>KRKIIYLASPYGFSQQQKTLLLPPIVRALEALGIEVWEPFARNNQIDFSQADWAYRVAQADLQDVKNCDGIFAVVNGTPPDEGVMVELGMAIALNKAIFLFRDDFRRCSDNERYPLNLMLFAGLPEIGWENYYYTSVDEIQSHDKALYKWLTGM[4x]

Here, we characterize the structure and function of a thermophilic dNDT, the protein from Chroococcidiopsis thermalis (CtNDT). Nucleoside 2′-deoxyribosyltransferase (dNDT) enzymes catalyze transglycosylation via a covalent 2′-deoxyribosylated enzyme intermediate with retention of configuration, having applications in the biocatalytic synthesis of 2′-deoxynucleoside analogues in a single step. The reaction catalyzed by dNDT proceeds via a ping-pong mechanism, with the formation of a 2′-deoxyribosyl-enzyme intermediate covalently linked to an active-site glutamate.13 Transglycosylation occurs in a stereospecific manner, preserving the anomeric carbon in the β configuration in the newly formed 2′-deoxyribonucleoside. As with other NDT enzymes, the active site of CtNDT is formed by residues from two monomers, and therefore, it is only fully formed in the dimer/tetramer.

Structures were obtained with the two potential transition-state analogues ImmH and DADmeH. Enzymes evolved to bind tightly to their cognate transition state and therefore to stable compounds that most closely mimic the charge distribution and geometry of that transition state. Based on Scheme 1 and considering 2′-deoxyribonucleside1 as a substrate, releasing nucleobase1 and generating a 2′-deoxyribosylated enzyme, ImmH would mimic an early transition state in which the distance between ribose C1′ and the nucleobase is ∼1.5 Å, while DADmeH would mimic a late transition state, since the presence of a methylene bridge between ribitol N1′ (which replaces C1′ in DADmeH) keeps the nucleobase at a distance of ∼3.0 Å from these groups. For ImmH, ΔH was −5.25 ± 0.07 kcal mol–1, −TΔS was −0.36 ± 0.14 kcal mol–1, and KD was 78.2 ± 6.6 μM, while for DADmeH, ΔH was −11.43 ± 0.29 kcal mol–1, −TΔS was 0.38 ± 0.73 kcal mol–1, and KD was 9 ± 5 nM. ΔG was −5.60 ± 0.08 for ImmH and −11.05 ± 0.42 kcal mol–1 for DADmeH; therefore, binding is determined by an enthalpic contribution. In the structure of bound DADmeH, however, E88 is 2.5 Å from N1′ in the sugar (analogous to C1′ in the substrate), 2.9 Å from Y7, and 3.5 Å from D62. D62 and Y7 are 3.4 Å apart. Stabilizing the nascent positive charge in the leaving group is D111, 2.5 Å away from Nitrogen 7 on DADmeH and 3.2 Å away from D62. The distance between D111 and N7 from DADmeH is shorter than the sum of the van der Waals radii for O and N, indicative of a very strong hydrogen bond between the two groups. Therefore, in the complex with DADmeH, E88 is closer to the bond that needs to be broken, D111 is closer to the nucleobase leaving group, and D62 is farther from interactions with the nucleobase when compared to an enzyme–substrate complex and also farther from the 3′-OH in comparison to the 2′-deoxyribosyl intermediate. This, coupled with the nM binding affinity of DADmeH for CtNDT, points toward a late transition state for the first half-reaction in which the bond order between sugar and nucleobase is negligible.>[4x]GSHMASKPIEDYGKGKGRIEPMYIPDNTFYNADDFLVPPHCKPYIDKILLPGGLVKDRVEKLAYDIHRTYFGEELHIICILKGSRGFFNLLIDYLATIQKYSGRESSVPPFFEHYV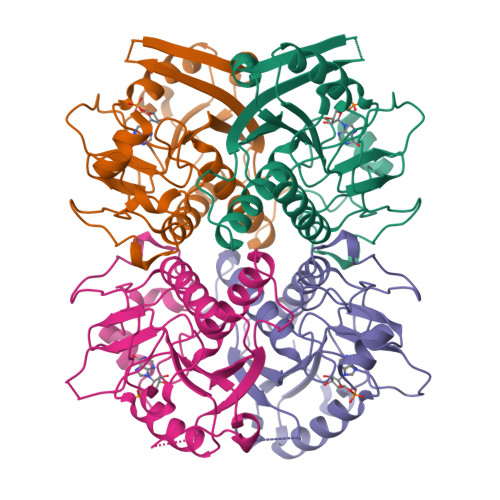RLKSYQNDNSTGQLTVLSDDLSIFRDKHVLIVEDIVDTGFTLTEFGERLKAVGPKSMRIATLVEKRTDRSNSLKGDFVGFSIEDVWIVGCCYDFNEMFRDFDHVAVLSDAARKKFEK>[2x]SHMTNLQTFELPTEVTGCAADISLGRALIQAWQKDGIFQIKTDSEQDRKTQEAMAASKQFCKEPLTFKSSCVSDLTYSGYVASGEEVTAGKPDFPEIFTVCKDLSVGDQRVKAGWPCHGPVPWPNNTYQKSMKTFMEELGLAGERLLKLTALGFELPINTFTDL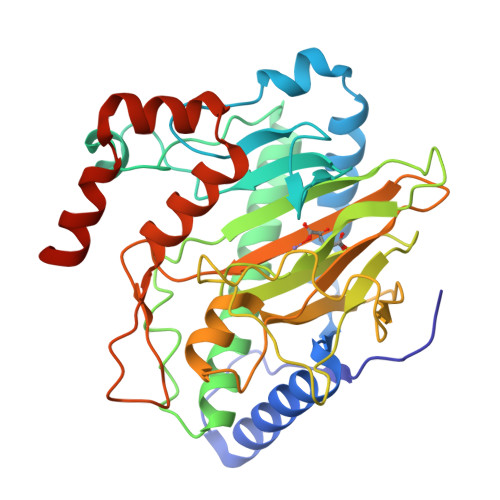TRDGWHHMRVLRFPPQTSTLSRGIGAHTDYGLLVIAAQDDVGGLYIRPPVEGEKRNRNWLPGESSAGMFEHDEPWTFVTPTPGVWTVFPGDILQFMTGGQLLSTPHKVKLNTRERFACAYFHEPNFEASAYPLFEPSANERIHYGEHFTNMFMRCYPDRITTQRINKENRLAHLEDLKKYSDTRATGS> IVGGSTIQPERVDAAALRQLGDAMRKVVGSADPTPLADLLSGTPVDPDELTREVGADGRQALLDSGMAVDDGTTFSSPLRGHQLHGVVVLSDPDVEEEVQHRWYVDPLWEADLLIRLMLRRGGARALDMGCGSGVLSLVLADRYESVLGVDVNPRAVALSRLNAALNGLTNVTFREGDMFEPAEGRFSRIVFNSPTNEEGNEFVDLLEAGEPILETFFRNVPRKLESGGIVEVNLAMNDYPGDPFRERL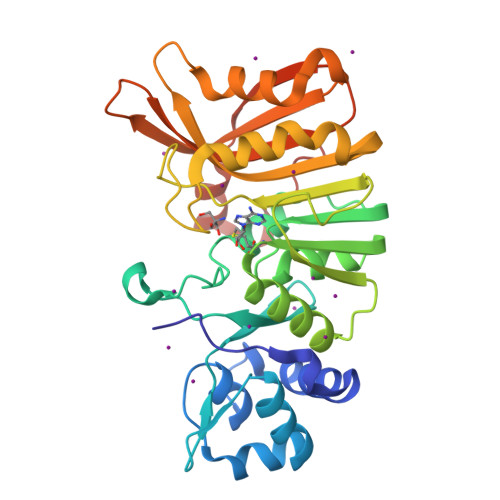ADWLGLTENGLRVQIFTSQRRATESGGEWKRGWLVVAPGPVGLTEVEWPYHDRYEEDPDALLDGTDRLLRG>[2x]RSPVFTDNSSPPAVPQSFQVAHLHAPTGSGKSTKVPAAYAAQGYKVLVLNPSVAATLGFGAYMSKAHGVDPNIRTGVRTITTGSPITYSTYGKFLADGGCSGGAYDIIICDECHSTDATSILGIGTVLDQAETAGARLVVLATATPPGSVTVSHPNIEEVALSTTGEIPFYGKAIPLEVIKGGRHLIF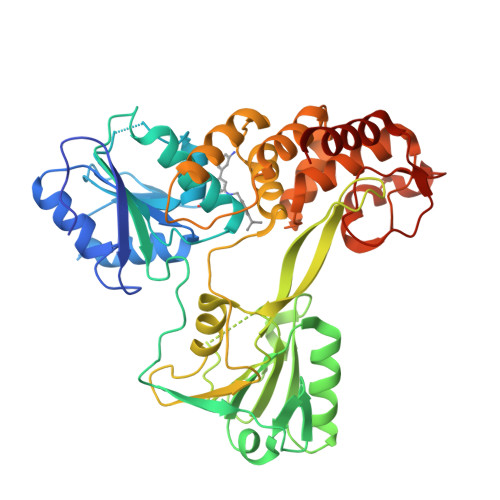CHSKKKCDELAAKLVALGINAVAYYRGLDVSVIPTSGDVVVVSTDALMTGFTGDFDSVIDCNTCVTQTVDFSLDPTFTIETTTLPQDAVSRTQRRGRTGRGKPGIYRFVAPGERPSGMFDSSVLCECYDAGCAWYELTPAETTVRLRAYMNTPGLPVCQDHLEFWEGVFTGLTHIDAHFLSQTKQSGENFPYLVAYQATVCARAQAPPPSWDQMWKCLIRLKPTLHGPTPLLYRLGAVQNEVTLTHPITKYIMTCMSADLEVV>MSLSEKEFAHLQTLLPKPPEHHPHYAFRFIDLFAGIGGIRRGFESIGGQCVFTSEWNKHAVRTYKANHYCDPATHHFNEDIRDITLSHQEGVSDEAAAEHIRQHIPEHDVLLAGFPCQPFSLAGVSKKNSLGRAHGFACDTQGTLFFDVVRIIDARRPAMFVLENVKNLKSHDKGKTFRIIMQTLDELGYDVADAEDNGPDDPKIIDGKHFLPQHRERIVLVGFRRDLNLKADFTLRDISECFPAQRVTLAQLLDPMVEAKYILTPVLWKYLYRYAKKHQARGNGFGYGMVYPNNPQSVTRTLSARYYKDGAEILIDRGWDMATGEKDFDDPLNQQHRPRRLTPRECARLMGFEAPGEAKFRIPV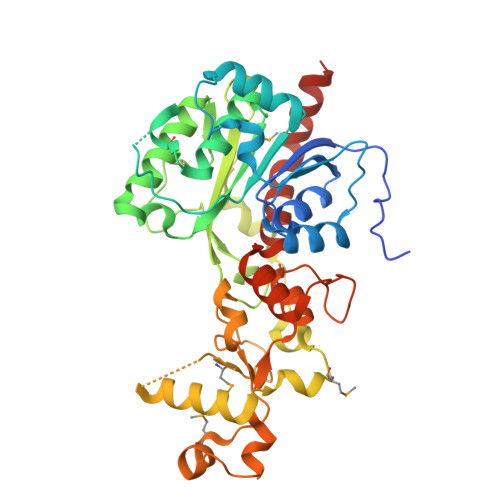SDTQAYRQFGNSVVVPVFAAVAKLLEPKIKQAVALRQEGHHHHHH[2x]> KG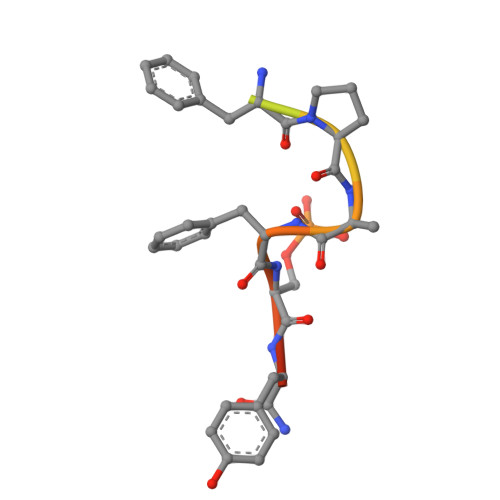AGGGGFPQFSYSA> MA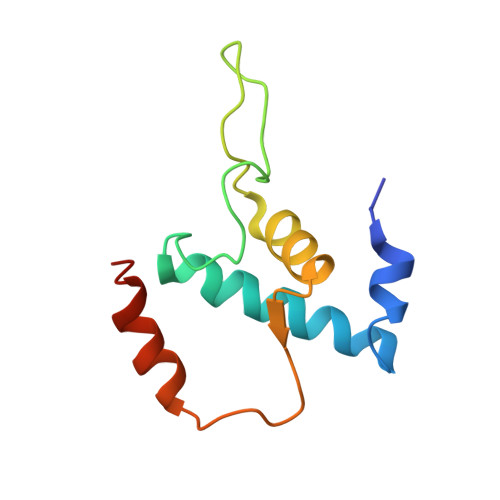EPGIDKLFGMVDSKYRLTVVVAKRAQQLLRHGFKNTVLEPEERPKMQTLEGLFDDPNAETWAMKELLTGRLVFGENLVPEDRLQKEMERIYPGEREE> MHHHHHHSSRENLYFQGTLPLWIGKPGDKPPPLCGAIPASGDYVARPGDKVAARVKAVDGDEQWILAEVVSYSHATNKYEVDDIDEEGKERHTLSRRRVIPLPQWKANPETDPEALFQKE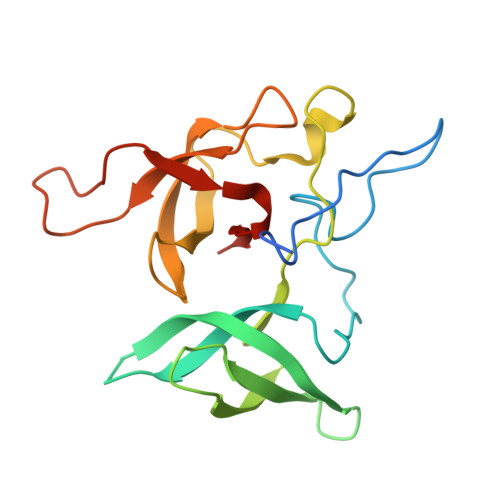QLVLALYPQTTCFYRALIHAPPQRPQDDYSVLFEDTSYADGYSPPLNVAQRYVVACKEPK> MGDNEEVKKMLEKMIEEIKKMLEKAIKKVKEMLEKMIKEIKKMLENGEDSEKILKKAKEMAEKILKMVIELAEKILKKAKEMAEKILKKVKELGVDNEEVKKMLEKMIEEIKKMLEK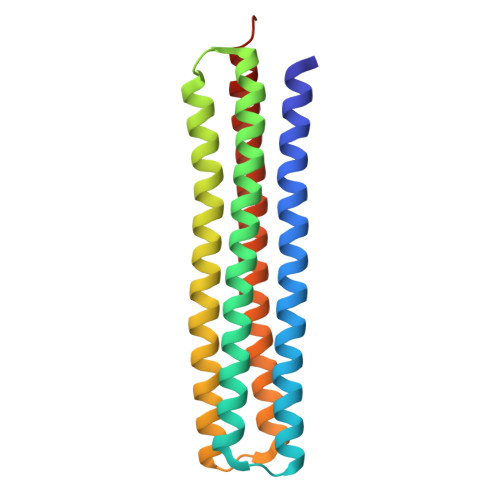AIKKVKEMLEKMIKEIKKMLENGEDSEKILKKAKEMAEKILKMVIELAEKILKKAKEMAEKILKKVKELGVGGW> HMWETLDDQRALQLALD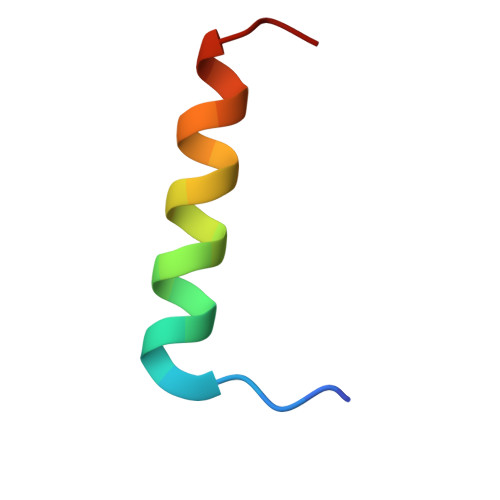QLSLLGL>MKIKQALFTAGYSSFYFDDQQAIKNGAGHDGFIYTGDPVTPGFTSVRQAGECVSVQLILENGAVAVGDCAAVQYSGAGGRDPLFLAEHFIPFLNDHIKPLLEGRDVDAFLPNARFFDKLRIDGNLLHTAVRYGLSQALLDATALASGRLKTEVVCDEWQLPCVPEAIPLFGQSGDDRYIAVDKMILKGVDVLPHALINNVEEKLGFKGEKLREYVRWLSDRILSLRSSPRYHPTLHIDVYGTIGLIFDMDPVRCAEYIA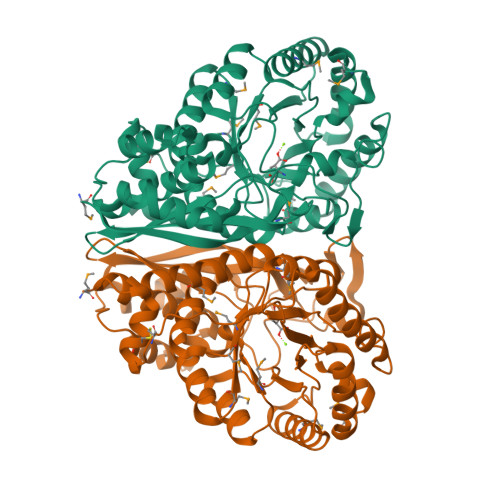SLEKEAQGLPLYIEGPVDAGNKPDQIRMLTAITKELTRLGSGVKIVADEWCNTYQDIVDFTDAGSCHMVQIKTPDLGGIHNIVDAVLYCNKHGMEAYQGGTCNETEISARTCVHVALAARPMRMLIKPGMGFDEGLNIVFNEMNRTIALLQTKD[2x]>GSMYVIRDEWGNQIWICPGCNKPDDGSPMIGCDDCDDWYHWPCVGIMTAPPEEMQWFCPKCANK[4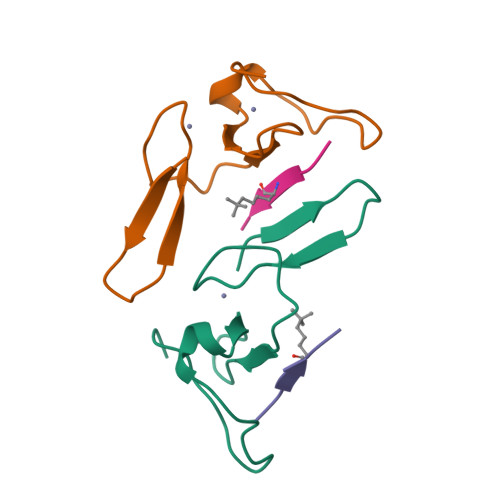x];>[4x]ARTXQTARKS>[2x]IVGGQECKDGECPWQALLINEENEGFCGGTILSEFYILTAAHCLYQAKRFKVRVGDRNTEQEEGGEAVHEVEVVIKHNRFTKETYDFDIAVLRLKTPITFRMNVAPACLPERDWAESTLMTQKTGIVS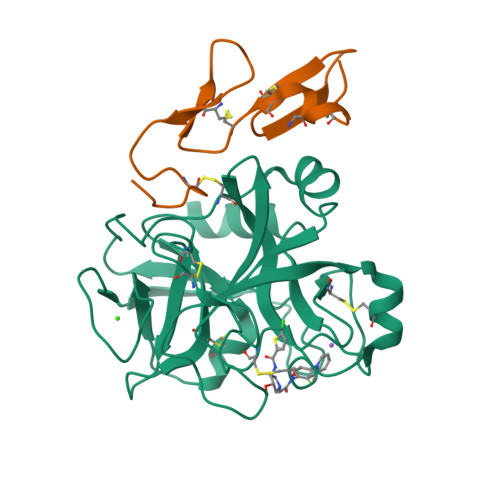GFGRTHEKGEQSTRLKMLEVPYVDRNSCKLSSSFIITQNMFCAGYDTKQEDACQGDSGGPHVTRFKDTYFVTGIVSWGEGCARKGKYGIYTKVTAFLKWIDRSMKTRGLPKAK;>RKLCSLDNGDCDQFCHEEQNSVVCSCARGYTLADNGKACIPTGPYPCGKQTLERR[2x]(5~{R})-7,8-dimethoxy-3,5-dimethyl-2,5-dihydro-1~{H}-3-benzazepin-4-one | C14 H19 N O3 | 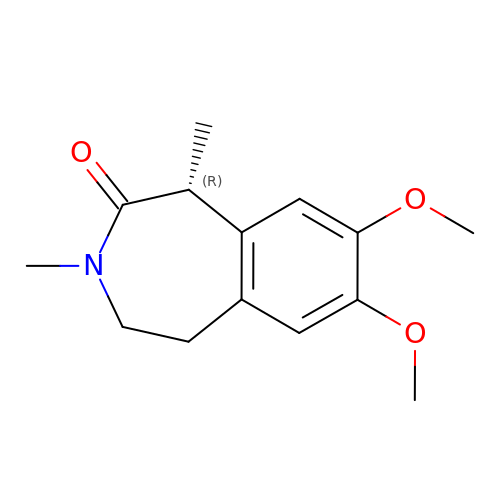PREGEFBQCOFCDI-SECBINFHSA-N(3R)-3-aminobutanamide 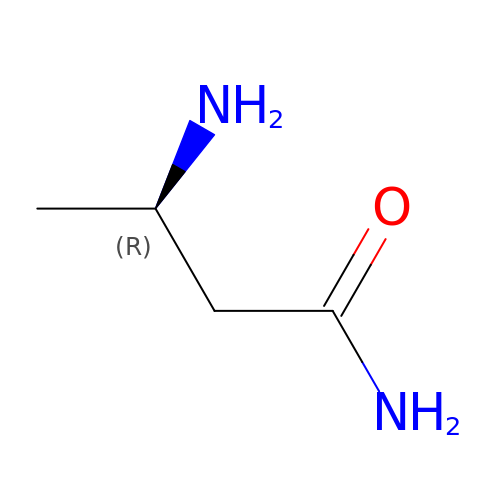| C4 H10 N2 O | OTVXVVYHNZUDSN-GSVOUGTGSA-N>MTTPQIDERAMEAGAAALQETIVDPGPLDVTALAVAAALAAGLHSAADDPAAALDKCIVLDELTEFAEKLVVHDRPGGIGTTVEYVEVYEDASGVRLGTATGNAVVLKMEPHMWQFHQSVSELADGSF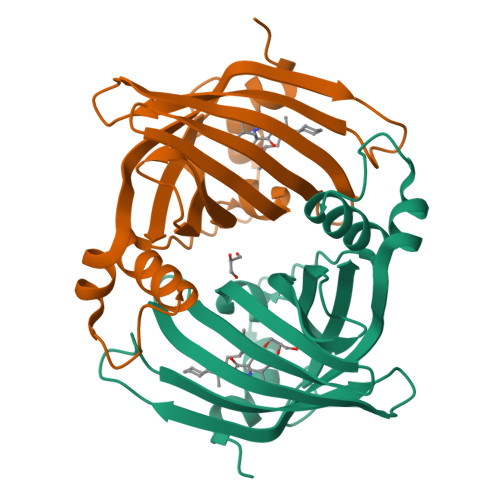EAVGVIDCTAMLRRMTQVLRVTGRSGRYAGKSGFMTLAISDPNQRPPHYSVQVVLC[4x]>MALIVQKFGGTSVGTVERIQAVAQRIKRTVQGGNSLVVVVSAMGKSTDVLVDLAQQISPNPCRREMDML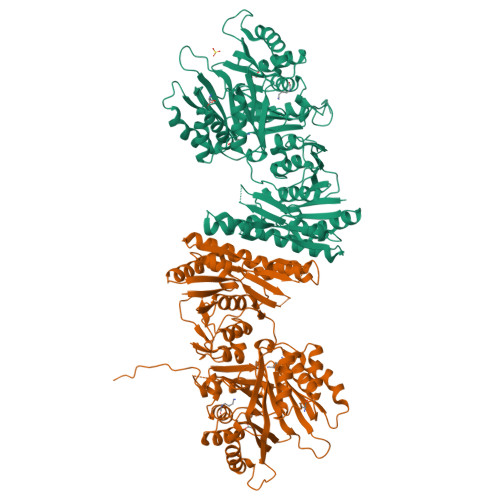LSTGEQVSIALLSLALQEIDQPAISLTGAQVGIVTEAEHSRARILEIRPDRLEHHLREGKVVVVAGFQGISSVEHLEITTLGRGGSDTSAVALAAALKADFCEIYTDVPGILTTDPRLVPEAQLMAEITCDEMLELASLGAKVLHPRAVEIARNYGIPLVVRSSWSDEPGTKVVAPPVQNRSLVGLEIAKAVDGVEYDADQAKVALLRVPDRPGVASKLFRDIAQQQVDIDLIIQSIHDGNSNDIAFTVVKDLLNTAEAVTSAIAPALRSYPEADQEAEIIVEKGIAKIAIAGAGMIGRPGIAAKMFKTLADVGVNIEMISTSEVKVSCVIDQRDADRAIAALSNAFGVTLSPPKNQTDTSHLPAVRGVALDQDQAQIAIRHVPDRPGMAAQLFTALAEANISVDMIIQSQRCRINQGTPCRDIAFMVAEGDSSQAEAILQPLIKDWLDAAIVVNKAIAKVSIVGSGMIGHPGVAAHFFAALAQENINIEMIATSEIKISCVVPQDRGVDALKAAHSAFNLAGTKTVTVPA[2x]>MKRKLIVAVVCLIFICFGINTPAHATSVVSIPINNAGFEDPFIEVVDDYTVDTPPGWTTYNPNNLVPEKRTTWTSNNGVGYVGPGTQFYNQLAPEGRNIGYIYLAQKPGSGVAGFEQILDATLEPDTNYTLKVDVGNLAGTFKGLSFAGFPGYRVELLAGDTVLAADHNNLFIKEGEFKTSTVTYTSTAKDLHLGQKLGIRLVNLLQD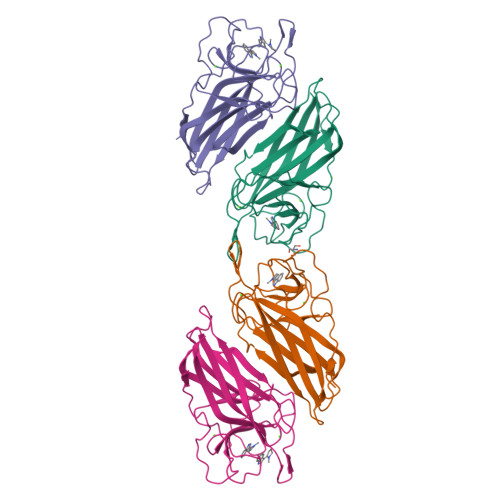KFSGLDFDNVRLTAEPTEA[4x]>GGSGGSYRVVAYYISWGAYGRSYFPSDIDYSKVTHINYAFANIKDGEVVVGDPGVDDGGKNNFTALRKAKKAHPHLRNLISVGGWSWSSGFSDAAATPEARKRFADSAVAFIRKYGFDGVDINWEYPVEGGAENMKHRPEDKQNYTLLTRSLREALDTAGKADGKYYELTTAVWGNDKFIANTEMDKVSRDFDFINVMSYDFNGTWNKFSGHNAPFVNDPAYDKPGIGKTFNVVSAVEAYLKAGVPADKLVVGVPLYGYSWKGCAAGERNGEYQDCNGKGRGTWEDGNLDFTDIEKNLLNKKGFKRYWNDTAKAAYLYNAETGEFVTYEDPQALKIKLDYIKSKGLGGAMYWEITADRKQTLVNLIADEL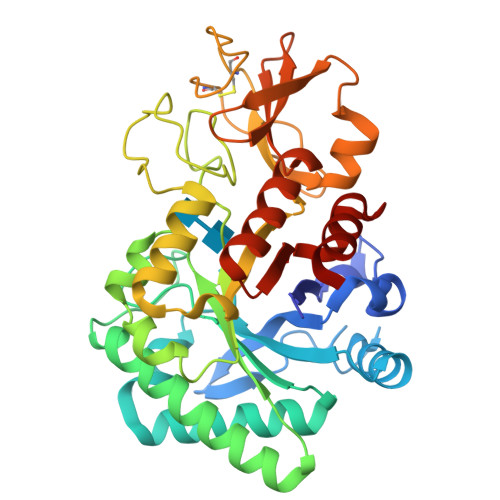LT[2x]1-methoxy-2-[2-[2-[2-[2-[2-[2-[2-[2-[2-(2-methoxyethoxy)ethoxy]ethoxy]ethoxy]ethoxy]ethoxy]ethoxy]ethoxy]ethoxy]ethoxy]ethane | C24 H50 O12 | 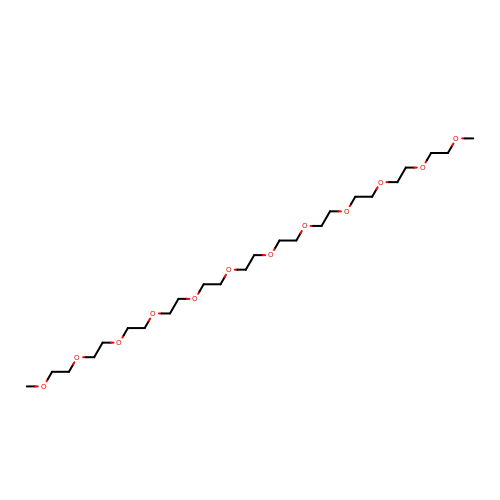WIQLMXVAXHHJSM-UHFFFAOYSA-N> EFETIERFMDCRIGRKGATGATTTIYAVEADGDPNAGFEKNKEPGEIQYLIKWKGWSHIHNTWETEETLKQQNVRGMKKLDNYKKKDQETKRWLKNASPEDVEYYNCQQELTDDLHKQYQIVERIIAHSNQKSAAGYP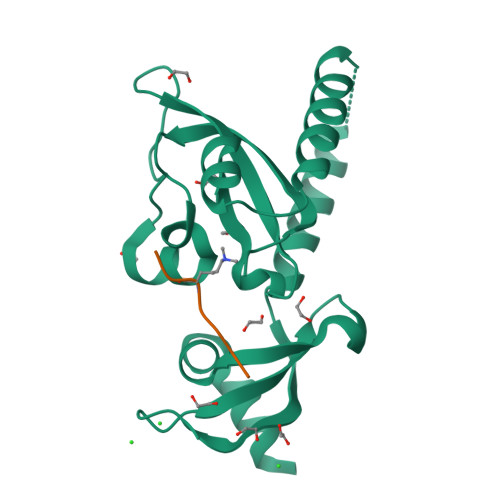DYYCKWQGLPYSECSWEDGALISKKFQACIDEYFSR;> RRTSRRKRAKVE> TKLHNTIFSETRKFTRESFKEIEHLTARLANDRVARHDFLFNTSIVLISDYSGEDSNGNQLQATITIPNEIINPKEYDPSDYPLAEDESFFKQGHKYDYLVTFRAGSLTNTYEPKTKMYKLHAALDKLMHVKQRKSRFADLWRELCAVIASLDVWYQTTNYPLRTYVKLLFHKGDEFPFYESPSQDRIIFNDKSVASILPTFVYTCCQVGTAIMSGILTHVESIVAMNHFLHCAKDSYIDEKLKIKGIGRSWYQEALHNVCQATVPVWSQFNEVIGHRTKSTSEPHFVSSTFISLRAKRAELLYPEFNAYINRAIQLSKTQNDVANYYAACRAMTNDGTFLATLTELSLDAAVFPRIEQHLVTRPAVLMSNTRHESLKQKYTNGVGSIAQSYLSSFTDEIAKRVNGRHHDEAWLNFLTTSSPGRKLTEIEKLEVGGDVAAWSNSRIVMQAVFAREYRTPERIFKSLKAPIKLVERQQSDRRQRAISGLDNDRLFLSFMPYTIGKQIYELNDNAAQGKQAGNAFDIGEMLYWTSQRNVLLSSIDVAGMDASVTTNTKDIYNTFVLDVASKCTVPRFGPYYAKNMEVFEAGNRQSQVRYVNAAWQACALEAANSQTSTSYESEIFGQVKNAEGTYPSGRADTSTHHTVLLQGLVRGNELKRASDGKNSCLATIKILGDDIMEIFQGSESDTYDHAVSNASILNESGFATTAELSQNSIVLLQQLVVNGTFWGFADRISLWTREDTKDIGRLNLAMMELNALIDDLVFRVRRPEGLKMLGFFCGAICLRRFTLSVDNKLYDSTYNNLSKYMTLTKYDKNPDSDSTLMSLILPLAWLFMPRGGEYPAYPFERRDGTFTEDESMFTARGAYKRRLLYDVSNIGEMIQQNSMALDDDLLHEYGFTGALLLIDLNILDLIDEVKKEDISPVKVSELATSLEQLGKLGEREKSRRAASDLKIRGHALSNDIVYGYGLQEKIQKSAMATKETTVQSKRVSSRLHDVIVAKTRDYKISTIPADALHLHEFEVEDVTVDLLPHAKHTSYSSLAYNMSFGSDGWFAFALLGGLDRSANLLRLDVAS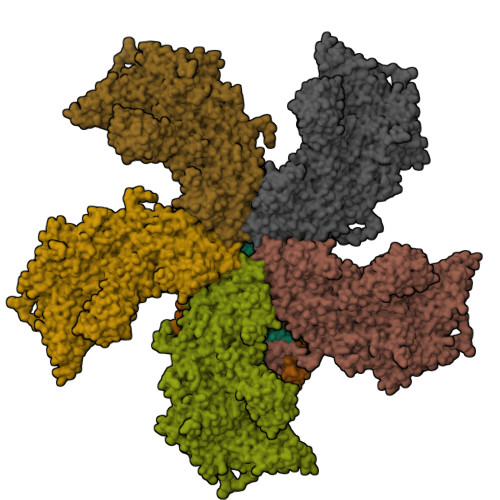IRGNYHKFSYDDPVFKQGYKIYKSDATLLNDFFTAISAGPKEQGILLRAFAYYSLYGNVEYHYVLSPRQLFFLSDNPVSAERLVRIPPKYYVSTQCRALYNIFSYLHILRSIANNRGKRLKMVLHPGLIAYVRG;> FAIDPLKHSKLYEEYGLYLRPHQINQEIKPTTIKKKELAPTIRSIKYASLIHSMLAEHAARHNGTLINPRMYADMITLGNTKVTVTKGTPKAQIDTLKMNGLTVVSKSRRNNKKKPVSDTTATIDENTNAIVTYKALTEMSTLIESFRLPSGLTLIIFDDEKYQSLIPNYINQLIAYTQPHIIPTWQGIADFSDTYLRSYFKRPFELTASNLAAPQKHNLSPMTRSIFNNTGREDAVIRKLYGYGEYVFIKYEGCLITWTGIYGEVTMMVNLSKRDLGLDVGDDYLKEYKKLLFYGVITDAIPSGISTRSTIMKISPHKMMNPSGGALAVLSKFLEAVVSTNVINATLVVYAEKGAGKTSFLSTYAEQLSLASGQVVGHLSSDAYGRWLAKTKDIEEPSFAYDYVLSLDTDDNESYYEQKASELLMSHGISEVAQYELLSVRKKIKMMDEMNEVLIAQLENADTHSERNFYYMVSTGKTTPRILIVEGHFNAQDATIARTDTTVLLRTINDTTQAMRDRQRGGVVQLFLRDTYYRLLPALHTTVYPFEMLESIKRWKWV;> VQSRTDVFNEQFANEALHPMTKVIFNGLDVNTEVQPLSDDFKQISDPKGYLTYSVKYEDQFTKKDKLRASEADDRIVGPTVNLFKYGAAVVNIDLNRDFFDTATGIDLTKGIPLVQDLLVPIGVTAGAEQSAEYVSGLLMVLFKVMTDNRLVIVGETTTPMSNTLSTVVNNVLRTTYHNNVGVNPALLRDFTQVNWLNRDITNMLQQAGTKYGLGLTETRLDYVRLVKTIVGHALNIDHFAASVLNINLRALMEANVTADDRIKALQAHSMISTQFHGPNQGALRPELAFDHDHIIRCLMLAAANYPRLEGIIVQINTGYVASANVIRPVSEKRYFPENLEQNQSAARLVSAVKARASEADISSIHLAIAREVSPMFNVHELKKIAESFEDPSSIVVVLEFILFALFFPTEFNRIKGDIQNVLLLFFSRWYPVEYGIFIQRGATYTINAAGEFEFSGRNEKWDQSLYLSEHFPALFSDVPLAGANTIIAIMRLFTPQGFLRTDDLAIAANFPRASRNPQTYIPYTNQRGTVTNEFASRFRTIVATLANVVNERAVQDDMQKATRSCTKQWLRHLETQFDNIAVAHTDHLSVVYATMSNFMLNFTNNFSGNHATFKPDQYVITSPEGSYKPIIERQGETVDGLTIIDTSIVWPILCQCTYPLVRQSGKGVDAVSIMEEIVYPDPSTTLSQSLSVAQVLSKLTLPDAFINMILSGGDSVVMRTYQTEADDDLDEGIRMTTYDQYLSHIRERLHITNVPDPIYITGASTPDQIAASVQATHVAVVLYQSGVINGSASTYLRENEVLVVMPDYYDVVSRFANANLQMNNNRYHESVLEIADIFDQADFIQTSDAVRQLRALMPTLSTSQIRHAIERIAQITDVDSTDYGKLTLRFLGTLTRSLKMQNAQIRRIRPDGTVLRYDDQIDIEAFRWSRYFLDELRLRRLSVGLRLITNPRIARRFDGVRIMYLTDDDPDPDFVPDVPEGYVAVQYAHRLFSSSLANKRNRVTYTHPPTGMAYPSPTGRPHVHMTINERAGMSKLVADNIIASVIKSNWVVDIHDIEYTAEVMTPSEGYTQHVDAESIMTAPKGKLFHLQFMDGLLRPEPSAFDPPASGEDMRLIYPLQPISVARSMRAIVNHNEVDRPRGAVAPSSYEMDTGTLSRNGDLLYSPVANGQVGIPKLEVDHISFSNVVSMMTANIRTGDDMAVERVNPDDVRAINIRNA;>[3x]ALHPMTKVIFNGLDVNTEVQPLSDDFKQISDPKGYLTYSVKYEDQFTKKDKLRASEADDRIVGPTVNLFKYGAAVVNIDLNRDFFDTATGIDLTKGIPLVQDLLVPIGVTAGAEQSAEYVSGLLMVLFKVMTDNRLVIVGETTTPMSNTLSTVVNNVLRTTYHNNVGVNPALLRDFTQVNWLNRDITNMLQQAGTKYGLGLTETRLDYVRLVKTIVGHALNIDHFAASVLNINLRALMEANVTADDRIKALQAHSMISTQFHGPNQGALRPELAFDHDHIIRCLMLAAANYPRLEGIIVQINTGYVASANVIRPVSEKRYFPENLEQNQSAARLVSAVKARASEADISSIHLAIAREVSPMFNVHELKKIAESFEDPSSIVVVLEFILFALFFPTEFNRIKGDIQNVLLLFFSRWYPVEYGIFIQRGATYTINAAGEFEFSGRNEKWDQSLYLSEHFPALFSDVPLAGANTIIAIMRLFTPQGFLRTDDLAIAANFPRASRNPQTYIPYTNQRGTVTNEFASRFRTIVATLANVVNERAVQDDMQKATRSCTKQWLRHLETQFDNIAVAHTDHLSVVYATMSNFMLNFTNNFSGNHATFKPDQYVITSPEGSYKPIIERQGETVDGLTIIDTSIVWPILCQCTYPLVRQSGKGVDAVSIMEEIVYPDPSTTLSQSLSVAQVLSKLTLPDAFINMILSGGDSVVMRTYQTEADDDLDEGIRMTTYDQYLSHIRERLHITNVPDPIYITGASTPDQIAASVQATHVAVVLYQSGVINGSASTYLRENEVLVVMPDYYDVVSRFANANLQMNNNRYHESVLEIADIFDQADFIQTSDAVRQLRALMPTLSTSQIRHAIERIAQITDVDSTDYGKLTLRFLGTLTRSLKMQNAQIRRIRPDGTVLRYDDQIDIEAFRWSRYFLDELRLRRLSVGLRLITNPRIARRFDGVRIMYLTDDDPDPDFVPDVPEGYVAVQYAHRLFSSSLANKRNRVTYTHPPTGMAYPSPTGRPHVHMTINERAGMSKLVADNIIASVIKSNWVVDIHDIEYTAEVMTPSEGYTQHVDAESIMTAPKGKLFHLQFMDGLLRPEPSAFDPPASGEDMRLIYPLQPISVARSMRAIVNHNEVDRPRGAVAPSSYEMDTGTLSRNGDLLYSPVANGQVGIPKLEVDHISFSNVVSMMTANIRTGDDMAVERVNPDDVRAINIRNA;> KKPPTVVQSRTDVFNEQFANEALHPMTKVIFNGLDVNTEVQPLSDDFKQISDPKGYLTYSVKYEDQFTKKDKLRASEADDRIVGPTVNLFKYGAAVVNIDLNRDFFDTATGIDLTKGIPLVQDLLVPIGVTAGAEQSAEYVSGLLMVLFKVMTDNRLVIVGETTTPMSNTLSTVVNNVLRTTYHNNVGVNPALLRDFTQVNWLNRDITNMLQQAGTKYGLGLTETRLDYVRLVKTIVGHALNIDHFAASVLNINLRALMEANVTADDRIKALQAHSMISTQFHGPNQGALRPELAFDHDHIIRCLMLAAANYPRLEGIIVQINTGYVASANVIRPVSEKRYFPENLEQNQSAARLVSAVKARASEADISSIHLAIAREVSPMFNVHELKKIAESFEDPSSIVVVLEFILFALFFPTEFNRIKGDIQNVLLLFFSRWYPVEYGIFIQRGATYTINAAGEFEFSGRNEKWDQSLYLSEHFPALFSDVPLAGANTIIAIMRLFTPQGFLRTDDLAIAANFPRASRNPQTYIPYTNQRGTVTNEFASRFRTIVATLANVVNERAVQDDMQKATRSCTKQWLRHLETQFDNIAVAHTDHLSVVYATMSNFMLNFTNNFSGNHATFKPDQYVITSPEGSYKPIIERQGETVDGLTIIDTSIVWPILCQCTYPLVRQSGKGVDAVSIMEEIVYPDPSTTLSQSLSVAQVLSKLTLPDAFINMILSGGDSVVMRTYQTEADDDLDEGIRMTTYDQYLSHIRERLHITNVPDPIYITGASTPDQIAASVQATHVAVVLYQSGVINGSASTYLRENEVLVVMPDYYDVVSRFANANLQMNNNRYHESVLEIADIFDQADFIQTSDAVRQLRALMPTLSTSQIRHAIERIAQITDVDSTDYGKLTLRFLGTLTRSLKMQNAQIRRIRPDGTVLRYDDQIDIEAFRWSRYFLDELRLRRLSVGLRLITNPRIARRFDGVRIMYLTDDDPDPDFVPDVPEGYVAVQYAHRLFSSSLANKRNRVTYTHPPTGMAYPSPTGRPHVHMTINERAGMSKLVADNIIASVIKSNWVVDIHDIEYTAEVMTPSEGYTQHVDAESIMTAPKGKLFHLQFMDGLLRPEPSAFDPPASGEDMRLIYPLQPISVARSMRAIVNHNEVDRPRGAVAPSSYEMDTGTLSRNGDLLYSPVANGQVGIPKLEVDHISFSNVVSMMTANIRTGDDMAVERVNPDDVRAINIRNA> ADQENSPLHTVGFDARFPQQNQTKHCWQSYVDYHKCVNMKGEDFA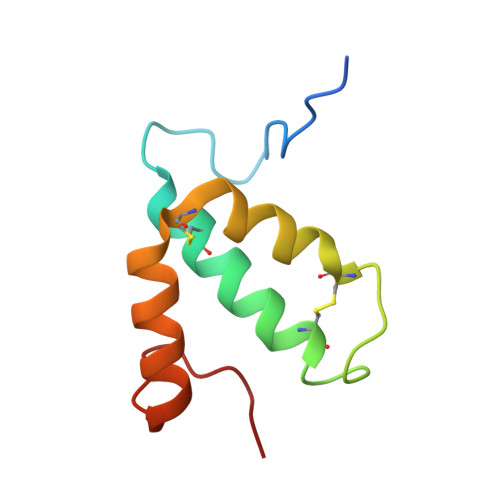PCKVFWKTYNALCPLDWIEKWDDQREKGIFAGDINSD> XEVNP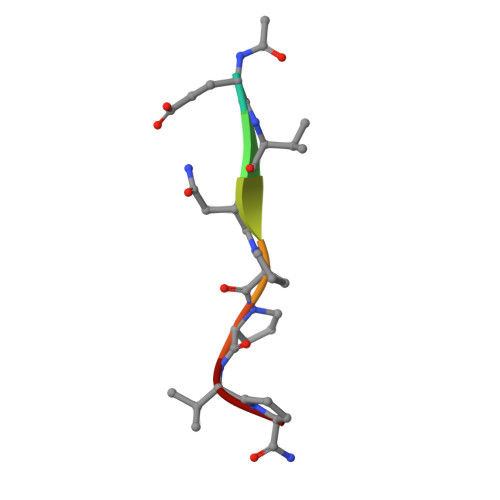PVP> SNAASGSALIFDEEMSRYKLLWTDPECEIEVPERLTVSYEALRTHGLAQRCKAVPVRQATEQEILLAHSEEYLEAVKQTPGMNVEELMAFSKKYNAVYFHQNIYHCAKLAAGATLQLVDSVMKREVRNGMALVRPPGHASQRSAANGFCVFNNVAFAALYAKKNYNLNRILIVDWDVHHGQGIQYCFEEDPSVLYFSWHRYEHQSFWPNLPESDYSSVGKGKGSGFNINLPWNKVGMTNSDYLAAFFHVLLPVAYEFDPELVIVSAGFDSAIGDPEGEMCALPEIFAHLTHLLMPLAAGKMCVVLEGGYNLTSLGQSVCQTVHSLLGDPTPRISGLGTACDSALESIQNVRNVQSSYWSSFKHLAQSETNPKRPRLDATNGGPKESSEPASESNPKKTAQDIVWPEPLKRMPASVRTVVVPPPGVELTLPKNCQHSGDISE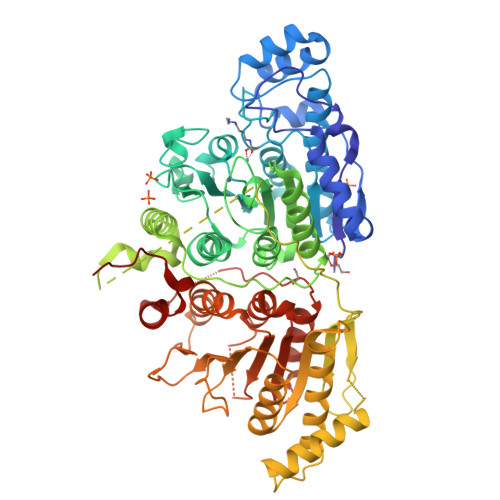STAKEVQRIRDKHFHDLTDQNILRSLGNIISVLDRMMRSDEVCNGCVVVSDLSVSVQCALQHALTEPAERVLVVYVGDGELPVKTNDGKVFLVQICTKETEDKCVNRLTLCLREGESLTAGFMQALLGLILPVAYEFNPALVLGIVEETAAKTRLMRVWGHMTCLIQGLARGRMLTLLQGYDKDLLELTVSALSGASISPLGPLRAPKPEDVEMMEKQRQRLQERWGLLRCTVSESW> GMATVILESIFLKRSQQKKKTSPLNFKKRLFLLTVQKLSYYEYDFERGRRGSKKGSIDVEKITCVETVVPEKNPPPERQIPRRGEESSETEQISIIERFPYPFQVVYDEGPLYVFSPTEELRKRWIHQLKNVIRYNSDLVQKYHPCFWIDGQYLCCSQTAKNAMGCQILAAAPSTAGLGYGSWEIDPKDLTFLKELGTGQFGVVKYGKWRGQYDVAIKMIKEGSMSEDEFIEEAKVMMNL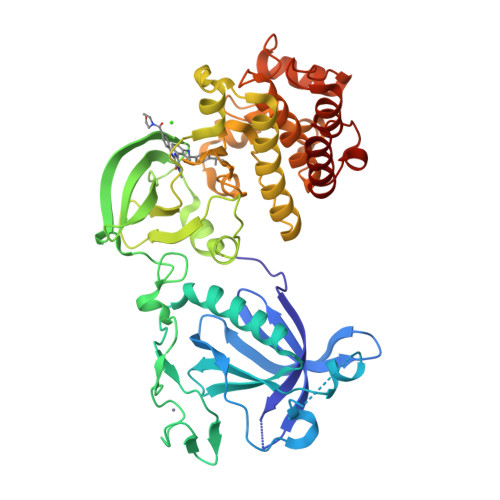SHEKLVQLYGVCTKQRPIFIITEYMANGCLLNYLREMRHRFQTQQLLEMCKDVCEAMEYLESKQFLHRDLAARNCLVNDQGVVKVSDFGMTRYVLDDEYTSSTGSKFPVKWASPEVLMYSKFSSKSDIWAFGVLMWEIYSLGKMPYERFTNSETAEHIAQGLRLPRPHLASERVYAIMYSCWHEKADERPTFKILLSNILDVMDEE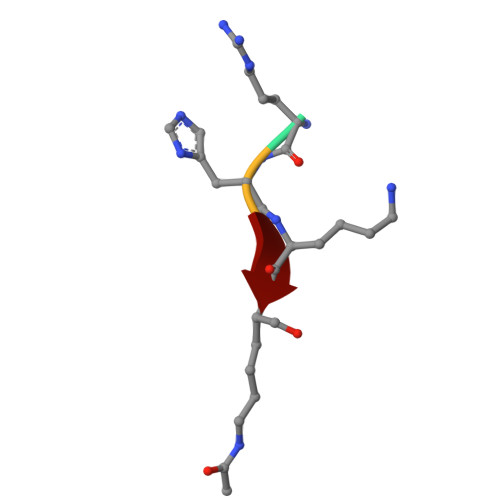> RHKK>MSLPRITAL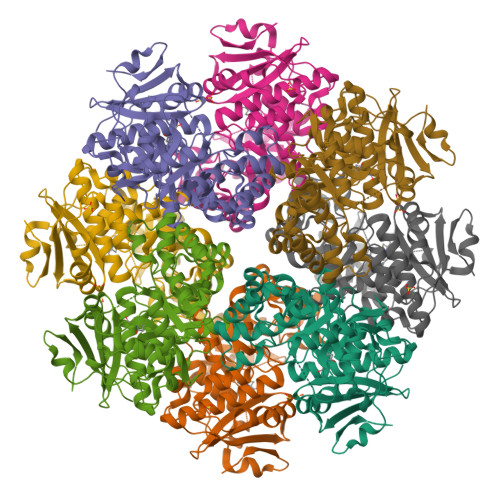RTIRLPERPKLIWVEVETEDGLTGLGETFRGAQAVEAVLHEQTAPAIIGRAAENITSISSELLNPYVGFGSSSAEVRAASAVDIALWDLAGQRAGVPLHVALGGAARDRVPVYATCAGYDFNTSLGGRRSIGSAELSTGPYDDQVAFMRDAGVLAESLVAEGYAAMKIWPFDDFASITPHHISLTDLKDGLEPFRKIRAAVGQRIEIMCELHSLWGTHAAARICNALADYGVLWVEDPIAKMDNIPAVADLRRQTRAPICGGENLAGTRRFHEMLCADAIDFVMLDLTWCGGLSEGRKIAALAETHARPLAPHDCTGPVALMAGLHLALHAPTAIFQEVVRASLATWYADLVDHLPVIQEGIALAPTRPGLGTALLPHVRKIAGAVVRESGKPREGHHHHHH[2x]>GSHMSAELEIDVKTRILDAAADAFMVHGFANTTIDDIAEQVGATKGLIYYHFRSKFDIFLAVYEDGMRRVRERVEPHAGGAGTGRERLVAMSVAHLENLMTELGYHHVVHQGVRYQASTALKIRQRDALAALNELRRDYELMFRRVVAEGIADGSLRVVDEALATRTLLSNLNAVDMWYRRIEGQTLDEINELATNVVDLLITGMANPQGRPR[4x]

The mycobacterial repressor, DarR, a TetR family regulator (TFR), was the first transcription regulator shown to bind c-di-AMP. Recently, DarR, a 201 residue, TFR regulator of a putative MDR transporter, Ms5347, in Mycobacteria was discovered and represents the focus of this work. Structures of TFR proteins reveal that they share a two-domain architecture with an N-terminal DNA-binding domain and a C-terminal inducer binding/dimerization domain. The DarR N-terminal domain consists of helices 1-3 and the dimer domain is comprised of helices α4-α9. In DarR, dimerization is mediated by helices α8 and α9, which interact with α8´ and α9´ (where the prime indicates the other subunit in the dimer) to form a four-helix bundle dimerization module.

Crystals of M. smegmatis DarR and M. baixiangningiae DarR were produced that diffracted to 3.56 Å and 1.60 Å resolution, respectively. The M. baixiangningiae DarR structure was solved by selenomethionine single wavelength anomalous diffraction (SAD) and refined to final Rwork/Rfree values of 18.5%/20.2% to 1.6 Å. This structure was then used to determine the M. smegmatis DarR structure. There are two M. smegmatis DarR dimers in the crystallographic asymmetric unit (ASU) and one DarR subunit in the M. baixiangningiae DarR structure. While the M. smegmatis and M. baixiangningiae DarR structures have essentially the same overall folds, the distances between their DNA-binding recognition helices differ (as measured by the distance between the two centrally located Tyr47 residues on each recognition helix). In M. baixiangningiae DarR the helices are separated by 50 Å while the distance between these helices of the M. smegmatis dimer is 41 Å. Analyses of the electron density in binding pockets in the M. smegmatis DarR structure showed water molecules. But there was no evident density for a ligand. The distance between HTH motifs in the DarR-DNA complex (39 Å) is similar to that between recognition helices observed in the M. smegmatis DarR structure (41 Å), supporting that the latter structure adopts a DNA-bound-like state.Selenophosphate synthetase (SEPHS) is a key enzyme in the Sec pathway, being responsible for catalyzing the formation of the active selenium donor for this reaction, selenophosphate, from selenide and ATP. Our group previously showed that trypanosomatids conserve only one selenophosphate synthetase, SEPHS2 (SPS2), containing a catalytic cysteine. Like E. coli SEPHS (SelD), but in contrast with its H. sapiens orthologs, trypanosomatid SEPHS2 is not a selenoprotein itself. In this paper, we focused on the trypanosomatid selenophosphate synthetase, a key enzyme in the selenocysteine pathway that is responsible for catalyzing the formation of the biological form of selenium, selenophosphate, for selenocysteine biosynthesis.

We determined the crystal structure of an N-terminally truncated selenophosphate synthetase from L. major (ΔN-LmSEPHS2) consisting of an AIRS-like fold also conserved in E. coli, A. aeolicus and H. sapiens orthologs. ΔN-LmSEPHS2 crystallized as a monomer in the asymmetric unit showing a typical aminoimidazole ribonucleotide synthetase (AIRS)-like fold, which consists of two α+β domains labeled N- and C-terminal AIRS (AIRS and AIRS_C, respectively) ranging from amino acid residues 74 to 190 and 204 to 384, respectively. The N-terminal AIRS domain folds into a six-stranded β-sheet flanked by two α-helices and one 310-helix, while the AIRS_C domain also presents a six-stranded β-sheet that is flanked by seven α-helices and one 310-helix. Similarly, the apo ΔN-LmSEPHS2 crystal structure lacks a 69-amino acid residues-long N-terminal region that includes a glycine-rich loop, where the conserved catalytic residues Cys46 and Lys49 are located. An elongated dimer model of ΔN-LmSEPHS2 was generated using PDBePISA as a likely quaternary structure, stable in solution with a 3230 Å2 buried surface. The dimerization surface occurs mainly between the β2 and β5 strands of adjacent monomers and is also stabilized by hydrophobic interactions between side chains, leading to the formation of an eight-stranded β-barrel. The dimeric structure of ΔN-LmSEPHS2 conserves two symmetrically arranged ATP-binding sites, formed along the interface between AIRS and AIRS-C domains in each monomer. Our dimeric model of LmSEPHS2 contains two equivalent unbound active sites in an open conformation prior to ATP and metal binding, similar to what is observed in the apo E. coli and A. aeolicus SEPHS structures. We showed that the crystallized construct (ΔN-LmSEPHS2) does not complement selenoprotein biosynthesis in SEPHS deficient E. coli WL400(DE3) strain, as expected due to the lack of catalytic residues.

> MSHKRPQSSAGESNGAVDLKTPRFDPVSLGLPAEFQLTDYTRLKGCSCKLPQPKLLALLQELSATPGQKDVGMDCSIVPLHHTNSKGEALFLVSTTDFFFPSVSDPFLQGQIGAANVLSDLYSMGIPDCDTMLMLLAASTEMDEHERLITTREIMKGFAERARLATTTVTGGQTVMNPWPLIGGVAMAVVSEAEMVRPTGLLCAGDILVLTKPLGCQVAVNLKQWLLRPSPLYEEAIAGHISPEEIEELYNMATDSMRRLNREGARLMRKHGAHGATDVTGFGILGHANNFGAAQAVGDAPRSLCLVLERLPMFKTAVAASKQMNDKYRLLEGYSAETSGGLLVAFPSTTAAAAFCAELTAVDGGCPSWIVGHVEDRATNAVDGVYARLKDGYEIVEV>GSQIPASEQETLVRPKPELLKLLKSVGAQKDTYTMKEVLFYLGQYIMTKRLYDEKQQHIVYCSNDL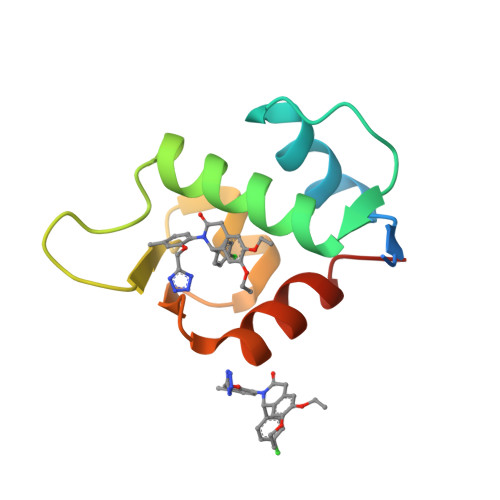LGDLFGVPSFSVKEHRKIYTMIYRNLVVVN[3x]>[6x]MAKVYKDLREFLEVLEQEGQLIRVKEEVNPEPDIAAAGRAAANLGKNQPAVFFEKIKGYKYSVVTNVHGSWQNHALMLGLDKNTSTKDQFYELNRRWDKFPVPPNVVKREAAPCKENVIDKDINLFEILPLYRINEQDGGFYISKASVVTADP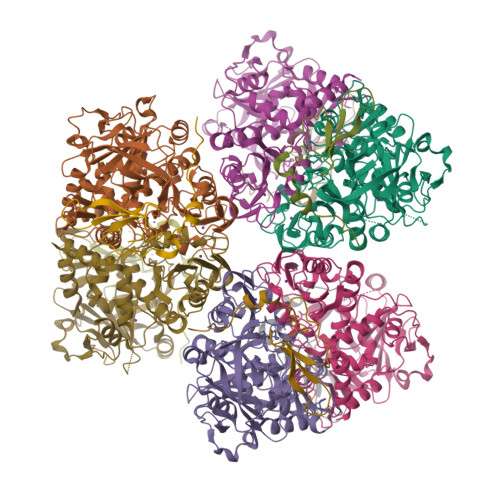EYPDDFNKLNVGTYRIQVKDRDRVGIQALAMHDIAVQLEKAEAENKPLPIAITIGNNPLVTFMASTPVGYNQNEYEFVGALQDGVPMDIVKSDLYDHLYVPAGSEVVLEGHIIPRVRTVEGPFGEFPGSYSGARLQCEVKIDRITHRTNPIFENLYLGIPWTEIDYLMALNTSVPLYKQLKETMPEVVAVNAMYTHGIGVIISTKVRYGGYAKGVAFRLLSTPHGMPYSKIVIVVDEFVDPFNLEQVMWALTTRVHPGKDVSIIENCPGMPLDPSTNPPGMHTKMIIDATTPVPPEPNPRETQLLDPPDGTEEWEEKLKELLKNQNR;>[6x]MKCHRCGSDNVRKMVDSPVGDAWEVYVCEKCCYSWRSTENPVVMEKFKLDDNKIANMGVIPPIPPLKK> GPLGSEIDYTAYPWFAGNMERQQTDNLLKSHASGTYLIRERPAEAERFAISIKFNDEVKH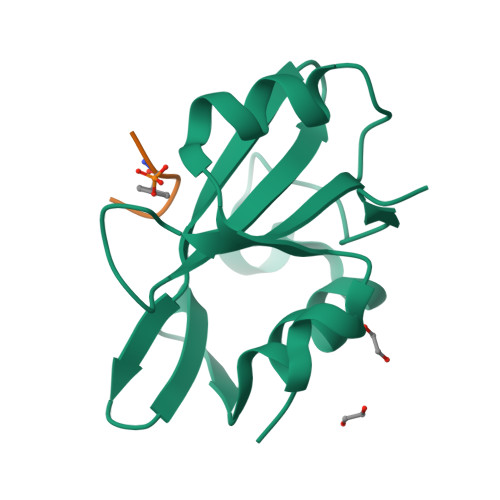IKVVEKDNWIHITEAKKFDSLLELVEYYQCHSLKESFKQLDTTLKYPYKSRERSAGIL;> KDSYVGDEA>[2x]GPLGSMAGTFKIHAYTEGGKPLRTIYLPKLLKKVFLDVVKPNTKKNLETCGILCGKLRQNAFFITHLVIPLQEATSDACGTTDEASLFEFQDKHNLLTLGWIHTHPTQTCFMSSVDLH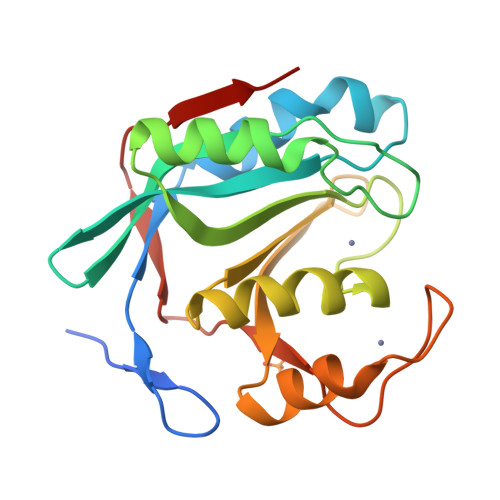THCSYQLMLPEAIAIVMAPSKNTSGIFRLLDPEGLQTIVKCRKPGLFHPHEGKVYTMVAQPGHVREINSKLQVVDLRVK> AKKETIDKVSDIVKEKLALGADVVVTADSEFSKLGADSLDTVEIVMNLEE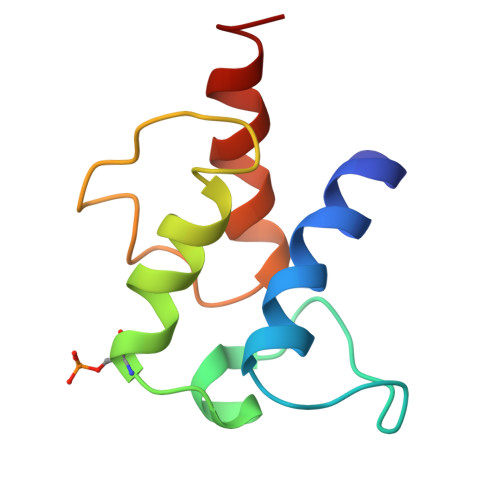EFGINVDEDKAQDISTIQQAADVIEGLLEKKA> GSAKDPKALSDFKTLE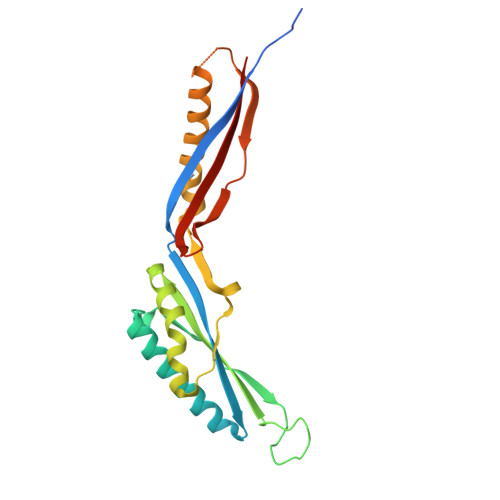RSVSVKGLSQKEVEADTLILPIKFTRSNNNLTNLYEELEQDKENIIKFLKEQGVKEDEINYNSPNIIDRLSDPYSNDTQAAYRYIGTANLLIYTQNVKLGKSILENISSLAKFGIVTKIDDYDIEYLYTKLNEIKPQMIEEATLNARNAAIKFAQDSNSHLGKIKKASQGQFSINNRDKNTPYIKTIRVVSTIEYYLKD5-ethyl-4-fluoro-2-(2-fluorophenoxy)phenol | C14 H12 F2 O2 | 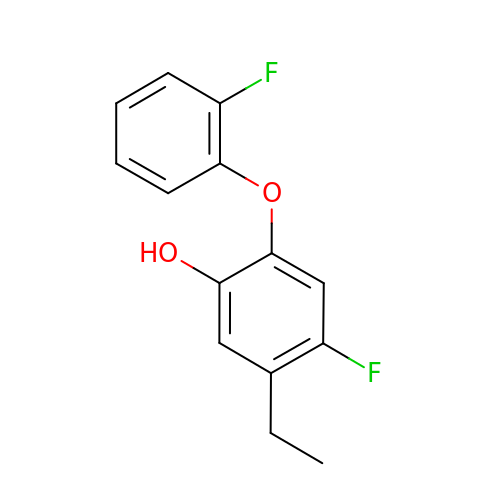MUHZCNPYLSMOCX-UHFFFAOYSA-N>MALFGYARVSTSQQSLDIQVRALKDAGVKANRIFTDKASGSSSDRKGLDLLRMKVKEGDVILVKKLDRLG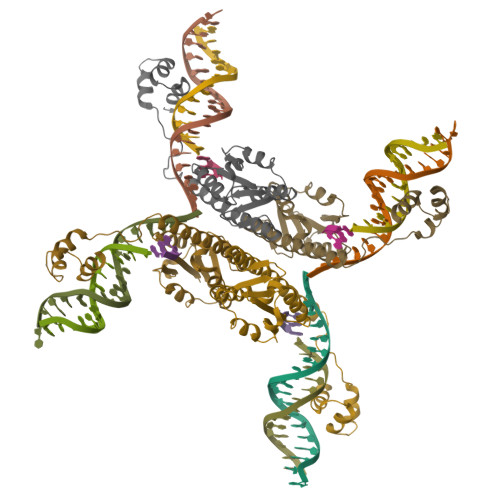RDTADMIQLIKEFDAQGVSIRFIDDGISTDSYIGKMVVTILSAVAQAERQRILQRTNEGRQEAMAKGVVFGRKRKIDRDAVLNMWQQGLGASHISKTMNIARSTVYKVINESN[4x]> AYTQQPGAPWGLGRISHRSKGSTTYEYDTSGGSGTCAYVIDTGVEASHPEFEGRASQIKSFISGQNTDGNGHGTHCAGTIGSKTYGVAKKTKIYGVKVLDNSGSGSYSGIISGMDFAVQDSKSRSCPKGVVANMSLGGGKAQSVNDGAAAMIRAGVFLAVAAGNDNANAANYSPASEPTVCTVGATTSSDARSSFSNYGNLVDIFAPGSNILSTWIGGTTNTISGTSMATPH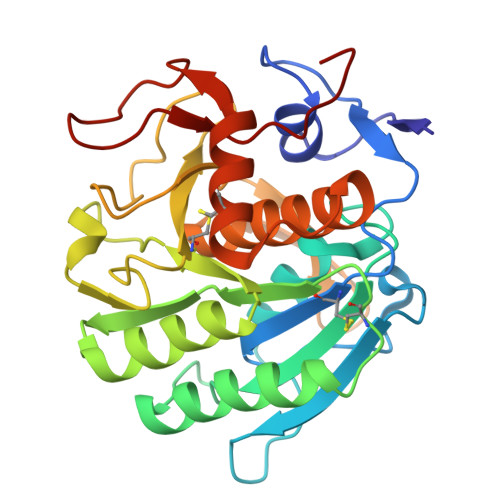IVGLGAYLAGLEGFPGAQALCKRIQTLSTKNVLTGIPSGTVNYLAFNGNPSG>[2x]MNRKWEAKLKQIEERASHYERKPLSSVYRPRLSKPEEPPSIWRLFHRQAQAFNFVKSCKEDVHVFALECKVGDGQRIYLVTTYAEFWFYYKSRKNLLHCYEVIPENAVCKLYFDLEFNKPANPGADGKKMVALLIEY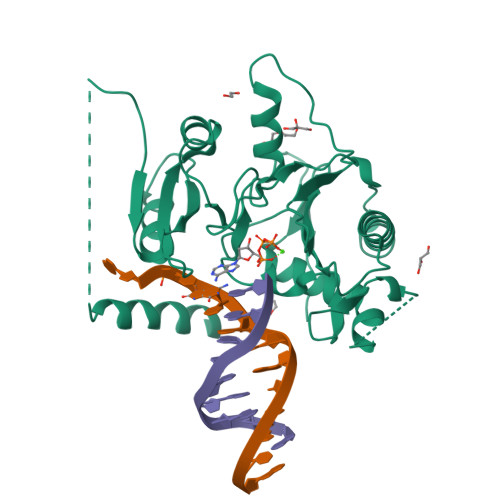VCKALQELYGVNCSAEDVLNLDSSTDEKFSRHLIFQLHDVAFKDNIHVGNFLRKILQPALDLLGSEDDDSAPETTGHGFPHFSEAPARQGFSFNKMFTEKATEESWTSNSKKLERLGSAEQSSPDLSFLVVKNNMGEKHLFVDLGVYTRNRNFRLYKSSKIGKRVALEVTEDNKFFPIQSKDVSDEYQYFLSSLVSNVRFSDTLRILTCEPSQNKQK> XVNAKQYHRILKRRQARAKLEAEGKIPKERX;> GPSFREQDIYLPIANVARIMKNAIPQTGKIAKDAKECVQECVSEFISFITSEASERCHQEKRKTINGEDILFAMSTLGFDSYVEPLKLYLQKFRE;> GPMEEIRNLTVKDFRVQELPLARIKKIMKLDEDVKMISAEAPVLFAKAAQIFITELTLRAWIHTEDNKRRTLQRNDIAMAITKFDQFDFLIDIV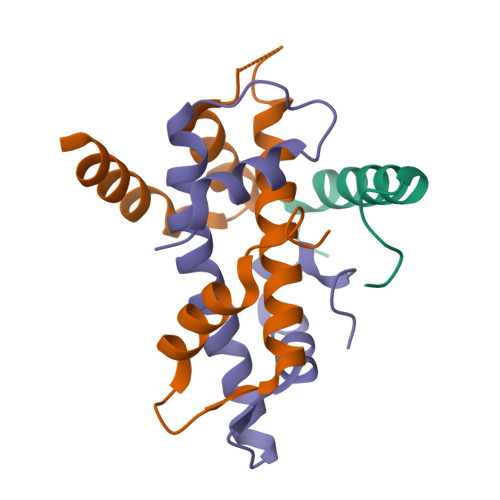PR>[4x]GHMSPNYDKWEMERTDITMKHKLGGGQYGEVYEGVWKKYSLTVAVKTLKEDTMEVEEFLKEAAVMKEIKHPNLVQLLGVCTREPPFYIITEFMTYGNLLDYLRECNRQEVNAVVLLYMATQISSAMEYLEKKNFIHRDLAARNCLVGENHLVKVADFGLSRLMTGDTYTAHAGAKFPIKWTAPESLAYNKFSIKSDVWAFGVLLWEIATYGMSPYPGIDLSQVYELLEKDYRMERPEGCPEKVYELMRACWQWNPSDRPSFAEIHQAFETMFQESSISDEVEKELGK;>[4x]AEEEIFGEFEAKK

BCR–Abl is a constitutively activated form of the nonreceptor tyrosine kinase c-Abl. The improper activation of the Abl tyrosine kinase results in chronic myeloid leukemia (CML). The recognition of an inactive conformation of Abl, in which a catalytically important Asp-Phe-Gly (DFG) motif is flipped by approximately 180° with respect to the active conformation, underlies the specificity of the cancer drug imatinib, which is used to treat CML. Our results suggest that interconversion between distinctly different inactive conformations is a characteristic feature of the Abl kinase domain.

We present a structure of the kinase domain of Abl, determined in complex with an ATP–peptide conjugate, in which the protein adopts an inactive conformation that resembles closely that of the Src kinases. Unexpectedly, one of these structures of the Abl kinase domain has a striking similarity to the conformation of inactive Src kinases (DFG-Asp In, αC-Glu Out). This is the first time that the same protein has been seen to adopt both the DFG-Asp Out and the αC-Glu Out inactive conformations. The conformation of molecule B is dramatically different from all other structures of Abl determined to date, all of which adopt the αC-Glu In conformation. The central result of this paper is the discovery that the kinase domain of Abl can readily adopt a conformation that resembles closely that of the inactive Src kinases. This is a surprise, because all previously seen conformations of the inactive forms of the Abl kinase domain have in common a flipped DFG motif (DFG-Asp Out/αC-Glu In), whereas the DFG motif is not flipped in the structures of the inactive Src kinases. We hypothesize, based on analysis of the structures in combination with targeted molecular dynamics simulations, that the DFG flip might be facilitated by adoption of the Src-like inactive structure. When helix αC is moved out of the active site, the DFG motif is freed from the steric hindrance imposed by the salt bridge between Glu 286 and Lys 271. The side chain of Phe 382 can then move through the sizable hydrophobic pocket created by the outward displacement of helix αC. Throughout the flip, the negative charge of Asp 381 is stabilized by the backbone amide groups of the activation loop and interaction with Arg 386.>[2x]AEVTQLSNGIVVATEHNPSAHTASVGVVFGSGAANENPYNNGVSNLWKNIFLSKENSAVAAKEGLALSSNISRDFQSYIVSSLPGSTDKSLDFLNQSFIQQKANLLSSSNFEATKKSVLKQVQDFEENDHPNRVLEHLHSTAFQNTPLSLPTRGTLESLENLVVADLESFANNHFLNSNAVVVGTGNIKHEDLVNSIESKNLSLQTGTKPVLKKKAAFLGSEVRLRDDTLPKAWISLAVEGEPVNSPNYFVAKLAAQIFGSYNAFEPASRLQGIKLLDNIQEYQLCDNFNHFSLSYKDSGLWGFSTATRNVTMIDDLIHFTLKQWNRLTISVTDTEVERAKSLLKLQLGQLYESGNPVNDANLLGAEVLIKGSKLSLGEAFKKIDAITVKDVKAWAGKRLWDQDIAIAGTGQIEGLLDYMRIRSDMSMMRW;>LTVSARDAPTKISTLAVKVHGGSRYATKDGVAHLLNRFNFQNTNTRSALKLVRESELLGGTFKSTLDREYITLKATFLKDDLPYYVNALADVLYKTAFKPHELTESVLPAARYDYAVAEQCPVKSAEDQLYAITFRKGLGNPLLYDGVERVSLQDIKDFADKVYTKENLEVSGENVVEADLKRFVDESLLSTLPAGKSLVSKSEPKFFLGEENRVRFIGDSVAAIGIPVNKASLAQYEVLANYLTSALSELSGLISSAKLDKFTDGGLFTLFVRDQDSAVVSSNIKKIVADLKKGKDLSPAINYTKLKNAVQNESVSSPIELNFDAVKDFKLGKFNYVAVGDVSNLPYLDEL[2x];>MAFRKSNVYLSLVNSYIIDSPQPSSINYWWNMGSLLGLCLVIQIVTGIFMAMHYSSNIELAFSSVEHIMRDVHNGYILRYLHANGASFFFMVMFMHMAKGLYYGSYRSPRVTLWNVGVIIFILTIATAFLGYCCVYGQMSHWGATVITNLFSAIPFVGNDIVSWLWGGFSVSNPTIQRFFALHYLVPFIIAAMVIMHLMALHIHGSSNPLGITGNLDRIPMHSYFIFKDLVTVFLFMLILALFVFYSPNTLGHPDNYIPGNPLVTPASIVPEWYLLPFYAILRSIPDKLLGVITMFAAILVLLVLPFTDRSVVRGNTFKVLSKFFFFIFVFNFVLLGQIGACHVEVPYVLMGQIATFIYFAYFLIIVPVISTIENVLFYIGRVNK[2x];>[2x]MTAAEHGLHAPAYAWSHNGPFETFDHASIRRGYQVYREVCAACHSLDRVAWRTLVGVSHTNEEVRNMAEEFEYDDEPDEQGNPKKRPGKLSDYIPGPYPNEQAARAANQGALPPDLSLIVKARHGGCDYIFSLLTGYPDEPPAGVALPPGSNYNPYFPGGSIAMARVLFDDMVEYEDGTPATTSQMAKDVTTFLNWCAEPEHDERKRLGLKTVIILSSLYLLSIWVKKFKWAGIKTRKFVFNPPKPRK;>[2x]KSTYRTPNFDDVLKENNDADKGRSYAYFMVGAMGLLSSAGAKSTVETFISSMTATADVLAMAKVEVNLAAIPLGKNVVVKWQGKPVFIRHRTPHEIQEANSVDMSALKDPQTDADRVKDPQWLIMLGICTHLGCVPIGEAGDFGGWFCPCHGSHYDISGRIRKGPAPLNLEIPAYEFDGDKVIVG;>MGMLELVGEYWEQLKITVVPVVAAAEDDDNEQHEEKAAEGEEKEEENGDEDEDEDEDEDDDDDDDEDEEEEEEVTDQLEDLREHFKNTEEGKALVHHYEECAERVKIQQQQPGYADLEHKEDCVEEFFHLQHYLDTATAPRLFDKLK[2x];>[2x]MPQSFTSIARIGDYILKSPVLSKLCVPVANQFINLAGYKKLGLKFDDLIAEENPIMQTALRRLPEDESYARAYRIIRAHQTELTHHLLPRNEWIKAQEDVPYLLPYILEAEAAAKEKDELDNIEVSK;>[2x]MGPPSGKTYMGWWGHMGGPKQKGITSYAVSPYAQKPLQGIFHNAVFNSFRRFKSQFLYVLIPAGIYWYWWKNGNEYNEFLYSKAGREELERVNV;>MSFSSLYKTFFKRNAVFVGTIFAGAFVFQTVFDTAITSWYENHNKGKLWKDVKARIAAGDGD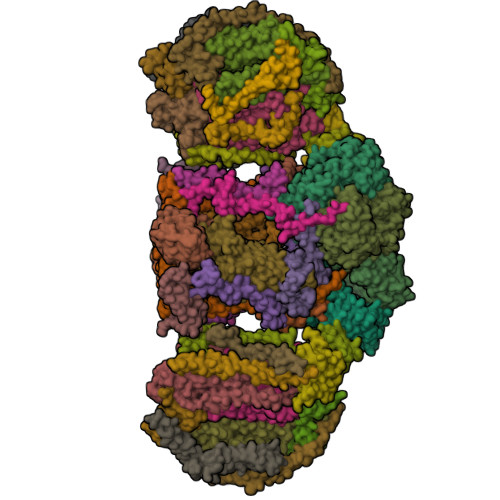DDDE[2x];>MAYTSHLSSKTGLHFGRLSLRSLTAYAPNLMLWGGASMLGLFVFTEGWPKFQDTLYKKIPLLGPTLEDHTPPEDKPN[2x];>MVQRWLYSTNAKDIAVLYFMLAIFSGMAGTAMSLIIRLELAAPGSQYLHGNSQLFNVLVVGHAVLMIFFLVMPALIGGFGNYLLPLMIGATDTAFPRINNIAFWVLPMGLVCLVTSTLVESGAGTGWTVYPPLSSIQAHSGPSVDLAIFALHLTSISSLLGAINFIVTTLNMRTNGMTMHKLPLFVWSIFITAFLLLLSLPVLSAGITMLLLDRNFNTSFFEVSGGGDPILYEHLFWFFGHPEVYILIIPGFGIISHVVSTYSKKPVFGEISMVYAMASIGLLGFLVWSHHMYIVGLDADTRAYFTSATMIIAIPTGIKIFSWLATIHGGSIRLATPMLYAIAFLFLFTMGGLTGVALANASLDVAFHDTYYVVGHFHYVLSMGAIFSLFAGYYYWSPQILGLNYNEKLAQIQFWLIFIGANVIFFPMHFLGINGMPRRIPDYPDAFAGWNYVASIGSFIATLSLFLFIYILYDQLVNGLNNKVNNKSVIYNKAPDFVESNTIFNLNTVKSSSIEFLLTSPPAVHSFNTPAVQS[2x];>[2x]DVPTPYACYFQDSATPNQEGILELHDNIMFYLLVILGLVSWMLYTIVMTYSKNPIAYKYIKHGQTIEVIWTIFPAVILLIIAFPSFILLYLCDEVISPAMTIKAIGYQWYWKYEYSDFINDSGETVEFESYVIPDELLEEGQLRLLDTDTSMVVPVDTHIRFVVTAADVIHDFAIPSLGIKVDATPGRLNQVSALIQREGVFYGACSELCGTGHANMPIKIEAVSLPKFLEWLNEQ;>MTHLERSRHQQHPFHMVMPSPWPIVVSFALLSLALSTALTMHGYIGNMNMVYLALFVLLTSSILWFRDIVAEATYLGDHTMAVRKGINLGFLMFVLSEVLIFAGLFWAYFHSAMSPDVTLGACWPPVGIEAVQPTELPLLNTIILLSSGATVTYSHHALIAGNRNKALSGLLITFWLIVIFVTCQYIEYTNAAFTISDGVYGSVFYAGTGLHFLHMVMLAAMLGVNYWRMRNYHLTAGHHVGYETTIIYTHVLDVIWLFLYVVFYWWGV[2x];>[2x]QQKPVVKTAQNLAEVNGPETLIGPGAKEGTVPTDLDQETGLARLELLGKLEGIDVFDTKPLDSSRKGTMKDPIIIESYDDYRYVGCTGSPAGSHTIMWLKPTVNEVARCWECGSVYKLNPVGVPNDDHHH;>[2x]VQTKALSKATLTDLPERWENMPNLEQKEIADNLTERQKLPWKTLNNEEIKAAWYISYGEWGPRRPVHGKGDVAFITKGVFLGLGISFGLFGLVRLLANPETPKTMNREWQLKSDEYLKSKNANPWGGYSQVQSK;>SDAHDEETFEEFTARYEKEFDEAYDLFEVQRVLNNCFSYDLVPAPAVIEKALRAARRVNDLPTAIRVFEALKYKVENEDQYKAYLDELKDVRQELGVPLKEELFPSSS[2x];>[2x]ANKVIQLQKIFQSSTKPLWWRHPRSALYLYPFYAIFAVAVVTPLLYIPNAIRGIKAKKA;>VHFKDGVYENIPFKVKGRKTPYALSHFGFFAIGFAVPFVACYVQLKKSGAF[2x];>[2x]TIAPITGTIKRRVIMDIVLGFSLGGVMASYWWWGFHMDKINKREKFYAELAERKK;>ADQENSPLHTVGFDARFPQQNQTKHCWQSYVDYHKCVNMKGEDFAPCKVFWKTYNALCPLDWIEKWDDQREKGIFAGDINSD[2x];>ASSLPPNALKPAFGPPDKVAAQKFKESLMATEKHAKDTSNMWVKISVWVALPAIALTAVNTYFVEKEHAEHREHLKHVPDSEWPRDYEFMNIRSKPFFWGDGDKTLFWNPVVNRHIEHDDGARGSHHHHHH[2x];>[2x]MFFSQVLRSSARAAPIKRYTGGRIGESWVITEGRRLIPEIFQWSAVLSVCLGWPGAVYFFSKARKA;>MKILTQDEIEAHRSHTLKGGIEGALAGFAISAIIFKVLPRRYPKFKPSTLTWSIKTALWITPPTVLTAICAEEASNNFDATMYGSGSSSEDALDEHRRWKSLSTKDKFVEGLSNNKYKIITGAWAASLYGSWVIVNKDPIMTKAQKIVQARMYAQFITVGLLLASVGLSMYENKLHPNKQKVNEMRRWENALRVAEEEERLEKEGRRTGYVSNEERINSKIFKS[2x]> MQ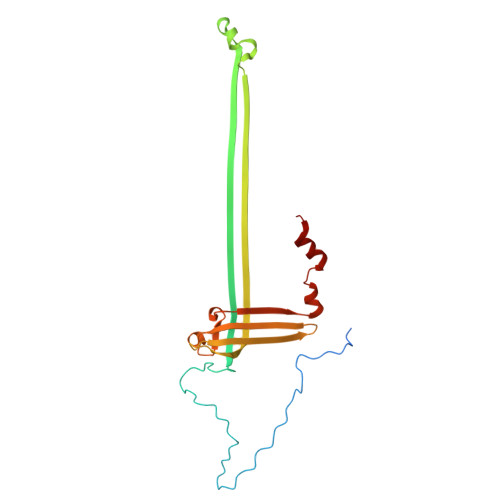KYALHAYPVMALMVATLTGCAWIPAKPLVQGATTAQPIPGPVPVANGSIFQSAQPINYGYQPLFEDRRPRNIGDTLTIVLQENVSASKSSSANASRDGKTSFGFDTVPRYLQGLFGNSRADMEASGGNSFNGKGGANASNTFSGTLTVTVDQVLANGNLHVVGEKQIAINQGTEFIRFSGVVNPRTISGSNSVPSTQVADARIEYVGNGYINEAQNMGWLQRFFLNLSPM>NNCPQDWLPMNGLCYKIFNELKAWKDAEMFCRKYKPGC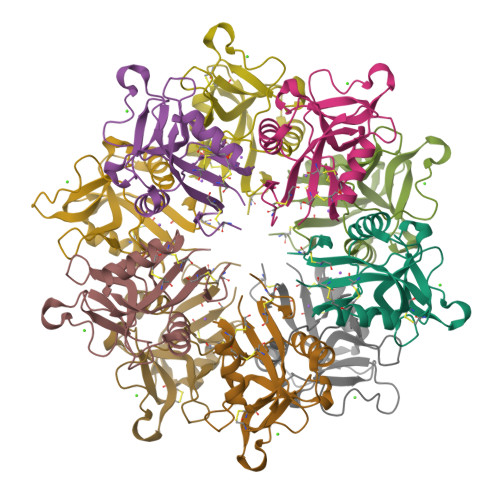HLASIHLYGESPEIAEYISDYHKGQSEVWIGLCDKKKDFSWEWTDRSCTDYLSWDKNQPDHYQNKEFCVELVSNTGYRLWNDQVCESKNAFLCQCKF[10x]>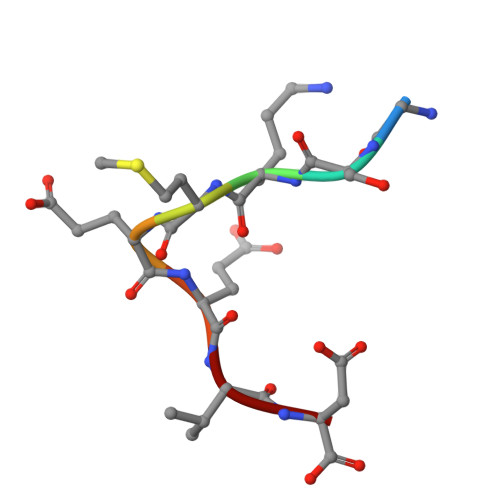 GSKMEEVD Proteins of the Ras superfamily of small GTPases regulate a variety of cellular processes such as intracellular transport, cell shape and motility, as well as differentiation and growth. For all of these processes, switching between the active GTP-bound and the inactive GDP-bound states is of fundamental importance. We describe here the synthesis of reactive acryl derivatives of guanine nucleotides that are able to react covalently with strategically placed cysteines in GTPases to lock them into their functional states in an irreversible manner. Extensive analysis of biochemical and structural features demonstrate the maintenance of the signalling ability of the modified GTPases.

Extending the labelling experiments to other GTPases, placing a cysteine at the position equivalent to E35 in Rab1b led to covalent interaction with aGTP for all those tested (Rab5A, Rab6A, Rab7A, Rab8A, Ypt7, HRas and Cdc42), albeit at variable rates, but substitution of cysteine at positions corresponding to L125 in Rab1b only led to covalent reaction in the case of Rab7A. Structural comparison of these adducts with Ypt7:GDP and Ypt7:GppNHp demonstrates that the covalent linker provides sufficient flexibility to allow the covalently locked proteins to adopt similar conformations of the nucleotide-binding pocket and in particular of the switch I region of Ypt7Q35C–aGDP, Ypt7Q35C–aGppNHp and Ypt7Q35C,K38I,Q68L–aGTP compared with the non-covalently nucleotide-bound proteins. Despite this flexibility, the electron density around the nucleotide and the linker was well defined in Ypt7Q35C–aGDP and Ypt7Q35C,K38I,Q68L–aGTP, whereas in Ypt7Q35C–aGppNHp this was only true for two (chains A and B) out of four copies within the asymmetric unit. In conclusion, the structures of Ypt7 modified with aGDP, aGTP or aGppNHp are very similar to the non-covalent Ypt7:nucleotide complexes, demonstrating that the structural properties of GTPases are maintained in covalently modified proteins. Additionally, covalent GTPase–nucleotide adducts also maintained the native structures and conformations, as demonstrated by the X-ray crystal structures of Ypt7Q35C–GDP, Ypt7Q35C–aGppNHp and Ypt7Q35C,K38I,Q68L–aGTP.

> GHMSSRKKNILKVIILGDSGVGKTSLMHRYVNDKYSCQYKATIGADFLTKEVTVDGDKVATMQVWDTAGQERFQSLGVAFYRGADCCVLVYDVTNASSFENIKSWRDEFLVHANVNSPETFPFVILGNKIDAEESKKIVSEKSAQELAKSLGDIPLFLTSAKNAINVDTAFEEIARSALQQNQA> AGKKRPWKCCDEAVC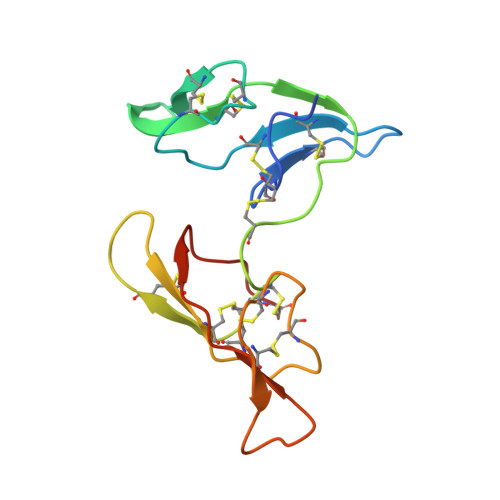TRSIPPICTCMDEVFECPKTCKSCGPSMGDPSRRICQDQYVGDPGPICRPWECCDKAICTRSNPPTCRCVDEVKKCAPTCKTCLPSRSRPSRRVCIDSYFGPVPPRCTPR>[3x]GPGSATTVHGETVVNGAKLTVTK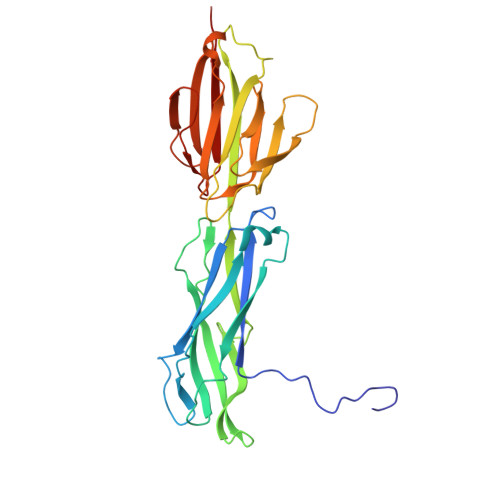NLDLVNSNALIPNTDFTFKIEPDTTVNEDGNKFKGVALNTPMTKVTYTNSDKGGSNTKTAEFDFSEVTFEKPGVYYYKVTEEKIDKVPGVSYDTTSYTVQVHVLWNEEQQKPVATYIVGYKEGSKVPIQFKNSLDSTTLTVKKKVSGTGGDRSKDFNFGLTLKANQYYKASEKVMIEKTTKGGQAPVQTEASIDQLYHFTLKDGESIKVTNLPVGVDYVVTEDDYKSEKYTTNVEVSPQDGAVKNIAGNSTEQETSTDKDMTITFTNKKVFE>[2x]MNGDCVDAKRVDTTDASKDGASASQPMQVDAKPQSHAFRYSLNYPNIGHCIIINNKNFDRRTGMNPRNGTDVDAGNVMNVFRKLGYIVKVYNDQTVAQIMQVLTTVAHDDHSRCASLVC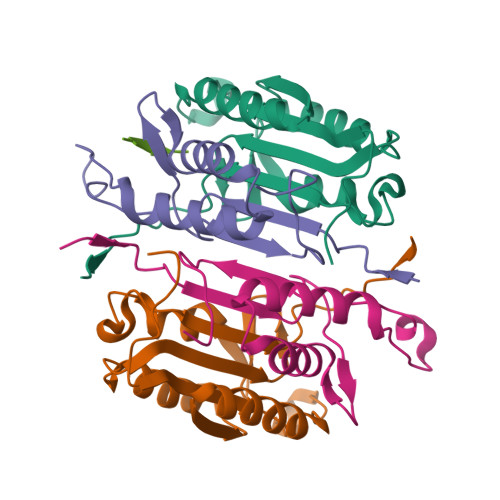VLLSHGDEGVFFGTDTSVDLKSLTSLFRGDRCPSLVGKPKLFFIQACRGTELDPGVETD;>[2x]RERIPVEADFLYAYSTVPGYYSWRTTMTGSWFIQSLCEMMTKYGSELELLQIMTRVNHKVALDFESTSNMPGFDAKKQIPCIVSMLTKEMYFTPLEHHHHHH;> DEVD4-methyl-N-{[(2R)-oxolan-2-yl]methyl}-1,3-thiazol-2-amine | C9 H14 N2 O S | 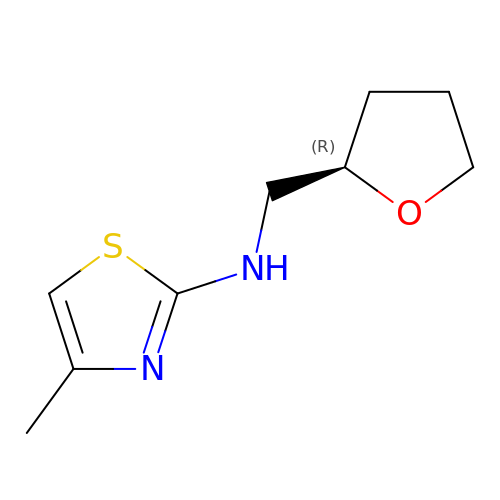VWLMRMKWLYRBMA-MRVPVSSYSA-N>MGRKIVFFDIDGTLLDEQKQLPLSTIEAVR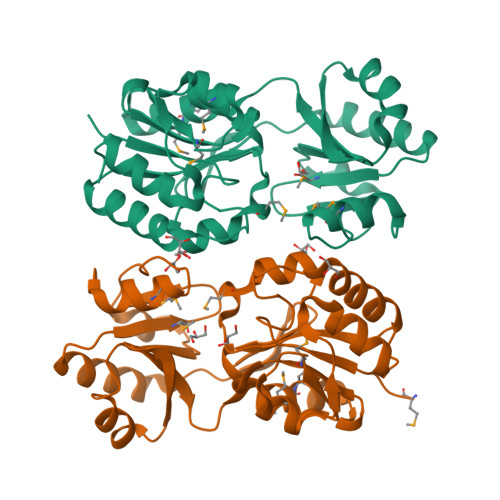RLKQSGVYVAIATGRAPFMFEHVRKQLGIDSFVSFNGQYVVFEGNVLYKQPLRREKVRALTEEAHKNGHPLVFMDAEKMRASIGDHPHIHVSMASLKFAHPPVDPLYYENKDIYQALLFCRAEEEEPYVRNYPEFRFVRWHDVSTDVLPAGGSKAEGIRMMIEKLGIDKKDVYAFGDGLNDIEMLSFVGTGVAMGNAHEEVKRVADFVTKPVDKEGIWYGLKQLQLIR[4x]Of particular interest is the Bdellovibrio bacteriovorus HD100 nucleoside diphosphate sugar (NDPS) hydrolase Bd3179 because it appears to have some of the characteristics of the Escherichia coli adenosine diphosphate ribose (ADPR) hydrolase and the guanosine diphosphate mannose (GDPM) hydrolase. Bd-NDPSase is a homodimer whose monomers are related by a non-crystallographic 2-fold axis. Each monomer comprises an N-terminal and a Nudix domain. Phosphate release assays revealed that among the nucleoside diphosphate sugars hydrolyzed by Bd-NDPSase, its highest relative activity was with GDPM.

The B-factor of the E140 Cα in apo Bd-NDPSase is 3.1 times larger than that of G115’ on loop L8, and 1.7 times larger than that of Y19 on loop L1, suggesting that loop L9 intrinsic flexibility facilitates substrate binding followed by E140 mediated nucleophilic attack of the scissile phosphate. A product-release mechanism where an arginine (R37 in Bd-NDPSase) completes a “fence” around the nucleoside is posible, but the presence of a sulfate ion in close proximity (4.5 Å) of R37 in the apo structure precludes this analysis.

>MKHLEEKTLSTRQIFKGRYLKIEQDQVQAPDGRTYTREYILHPGAAMMIPLLPNGNVVMIHQYRHAVKKVFLEFPAGKRDHNEETLLTAKRELLEETGYEAKDWKFLTTIHPVIGYSNEHIDLYLARDLTHLEQRLDQGEFIEVVEVKPADLMQLVLEGKVSDVKTQIGAFWLDKFLRGEWN[2x]> GEFTQSVSRLQSIVAGLKNAPSDQLINIFESCVRNPVENIMKILKGIGET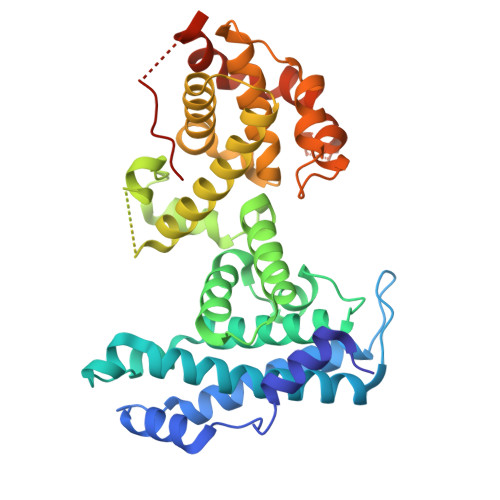FCQHYTQSTDEQPGSHIDFAVNRLKLAEILYYKILETVMVQETRRLHGMDMSVLLEQDIFHRSLMACCLEIVLFAYSSPRTFPWIIEVLNLQPFYFYKVIEVVIRSEEGLSRDMVKHLNSIEEQILESLAWSHDSALWEALQVSANKVPTCEEVIFPNNFETGNNRPKRTGSLALFYRKVYHLASVRLRDLCLKLDVSNELRRKIWTCFEFTLVHCPDLMKDRHLDQLLLCAFYIMAKVTKEERTFQEIMKSYRNQPQANSHVYRSVLLKSIKEERGDLIKFYNTIYVGRVKSFALKYDLANQDHMMDAPPLSPFPHIKQQ>EGDIHMKKGHHHHHHENLYFQGGSGKLSEQLKHCNGILKELLSKKHAAYAWPFYKPVDASALGLHDYHDIIKHPMDLSTVKRKMENRDYRDA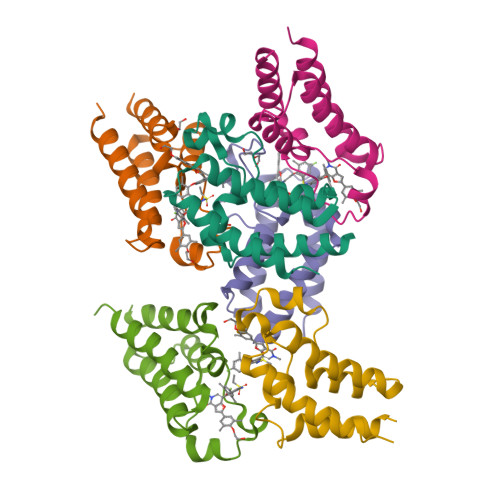QEFAADVRLMFSNCYKYNPPDHDVVAMARKLQDVFEFRYAKMPD[6x]> SSQIRQNYSTEVEAAVNRLVNLYLRASYTYLSLGFYFDRDDVALCGVAHFFRELAEEKREGAERLLKMQNQRGG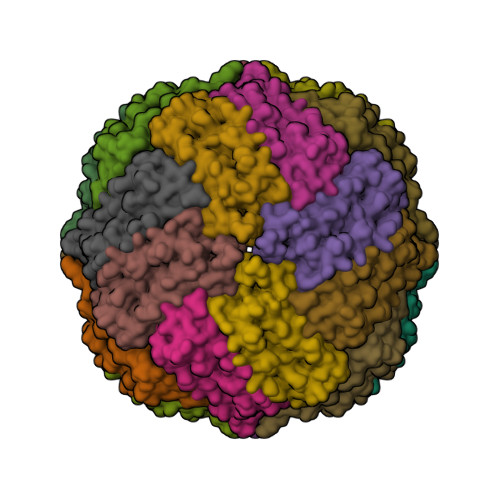RALFQDLQKPSQDEWGTTLDAMKAAIVLEKSLNQALLDLHALGSAQADPHLCDFLESHFLDEEVKLIKKMGDHLTNIQRLVGSQAGLGEYLFERLTLKHD> MVLGKVVGTVVASRKEPRIE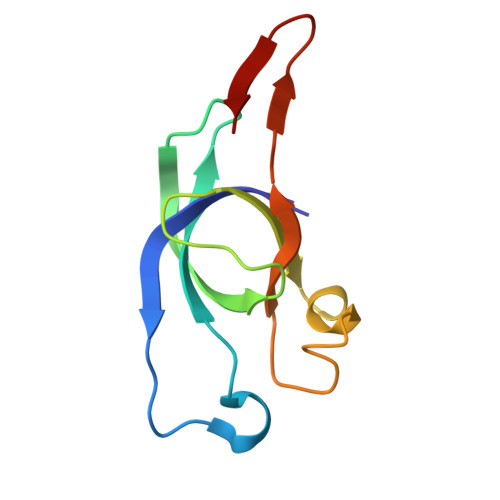GLSLLLVRACDPDGTPTGGAVVCADAVGAGVGEVVLYASGSSARQTEVTNNRPVDATIMAIVDLVEMGGDVRFRKD>MADSNLNEPVIIQATRLDTSILPRNIFSQSYLLYVIAQGTDVGNVANKANEAGQGAYDAQVKNDEQDVELADHDARIAANTKAINILEVRLTTAEGKIVVLRSDVDYLLDEVIDIQAHLVTVDQRLDGVESDVSDIKSDYVSKTVTESQSLASPLDVKTSYSVDGIQVVGARQTGWTAATGTPLLG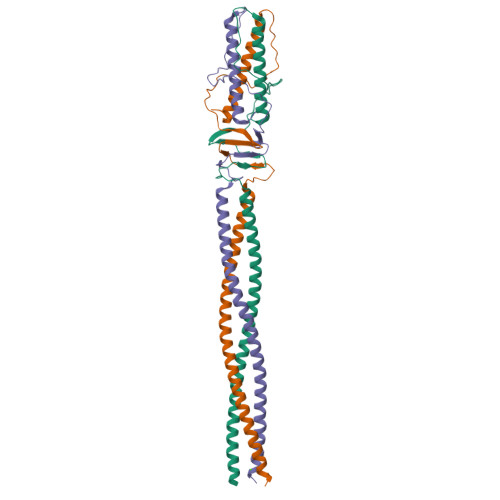SFNANQSYTVGTTYTQSEVAALATGLEQARQRILALETALRLHGLID[6x]> MHHHHHHHHPDLGTGSENLYFQGAMGKILLLGPERKWLRDFLESFEDEVTQY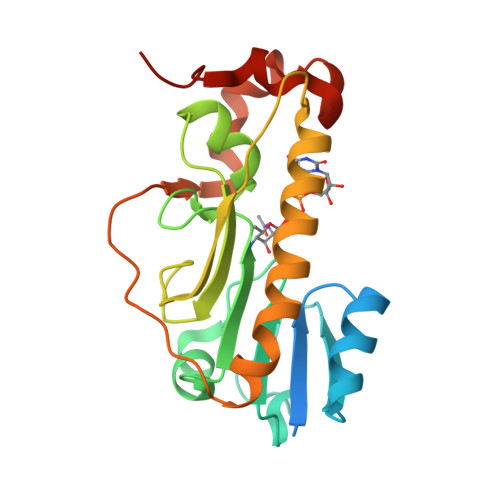QDKLDKKSAILNNVDFIISYGYRYIIHPDIVERFKQRAINLHISYLPWNKGADPNLWSFLEDSPKGVTIHYIDSGLDTGEIIVQREVTYYENDTLRTTYERLTQTIEKLFMEYWPLIRLGKIRGIPQPKGGSYHKLKDKEKYLYLLTDGWDTPVQKLIGKAQNNE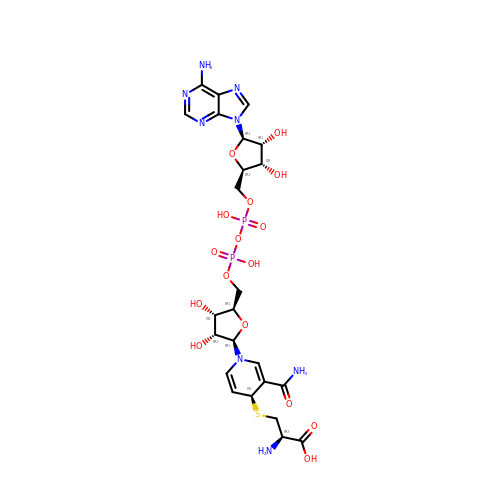(2R)-3-[[(4S)-3-aminocarbonyl-1-[(2R,3R,4S,5R)-5-[[[[(2R,3S,4R,5R)-5-(6-aminopurin-9-yl)-3,4-bis(oxidanyl)oxolan-2-yl]methoxy-oxidanyl-phosphoryl]oxy-oxidanyl-phosphoryl]oxymethyl]-3,4-bis(oxidanyl)oxolan-2-yl]-4H-pyridin-4-yl]sulfanyl]-2-azanyl-propanoic acid | C24 H34 N8 O16 P2 S | VVCRIRHVXHQAHX-VJDLECKTSA-N>GSGERKISRIHLVSEPSITHFLQVSWEKTLESGFVITLTDGHSAWTGTVSESEISQEADDMAMEKGKYVGELRKALLSGAGPADVYTFNFSKESCYFFFEKNLKDVSFRLGSFNLEKVENPAEVIRELICYCLDDLSQLQTEVEEAVQECRNAE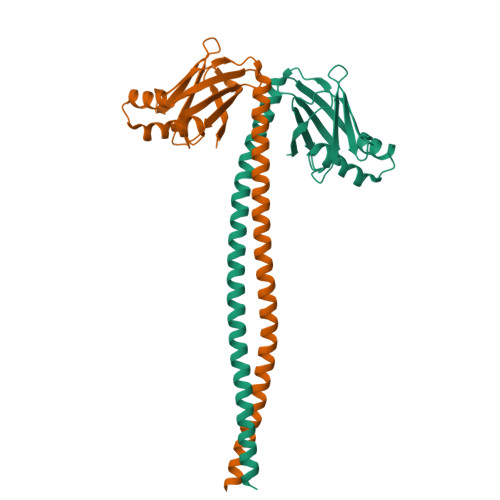EKAKKAITDAAMMAEELKKEQDTSAHLERMKKNMEQTIKDLQHRL[2x]> ATFEIVNRCSYTVWAAASKGDAALDAGGRQLNSGESWTINVEPGTNGGKIWARTDCYFDDSGSGICKTGDCGGLLRCKRFGRPPTTLAEFSLNQYGKDYIDISNIKGFNVPMDFSPTTRGCRGVRCAADIVGQCPAALKAPGGGCNDACTVFQTSEYCCTTGKCGPTEYSRFFKRLCPDAFSYVLDKPTTVTCPGSSNYRVTFCPTA

Among the sweet-tasting proteins, thaumatin is ~100,000 times sweeter than sucrose on a molar basis and about 1,600 times sweeter on a weight basis. The intensely sweet taste of thaumatin has been widely used not only as a natural sweetener, but also as a flavor enhancer and for masking unpleasant tastes in the food and pharmaceutical industries. Site-directed mutagenesis studies revealed that six lysine residues of Lys19, Lys49, Lys67, Lys106, Lys163, and Lys187, and three arginine residues of Arg76, Arg79, and Arg82 located on the cleft-containing side are responsible for sweetness, and two amino acids residues, Lys67 and Arg82, are particularly important for sweetness. In the present study, three mutant X-ray crystallographic structures of thaumatin (K78A, K106A, and K137A) were determined at resolutions of 1.07, 1.07 and 1.01 Å, respectively.

The final model of K137A thaumatin was determined at a slightly higher resolution of 1.01 Å. It consists of 3,309 protein atoms, including hydrogen atoms, 10 tartrate atoms, 18 glycerol atoms and 363 water molecules. Compared to K78A, K106A, and recombinant thaumatin, one tartrate molecule was reduced in K137A. The threshold values of K78A and K137A were 220 and 230 nM, respectively, and sweetness decreased by ~5-fold when compared to recombinant and plant thaumatin. In Lys137 of recombinant thaumatin, the B-factors of the main-chain and side-chain were 9.33 and 32.24 Å2, respectively. The normalized B-factor ratios of Ala137 were 1.00 for main-chain and 1.18 for side-chain, and those of Lys137 in recombinant thaumatin for main-chain and side-chain were 0.95 and 2.27, respectively. The normalized B-factor ratio decreased by 1.09 for side-chain, suggesting that the flexibility of the side-chain of Lys137 was substantially reduced. The reduction of flexibility at the interaction sites indeed seems to be consistent with the difference in sweetness, since the threshold value of K137A (230 nM) and K78A (220 nM) is higher than that of K106A (140 nM). The superposition between K137A and recombinant thaumatin showed no obvious differences in r.m.s.d. values except alternative side-chains and C-terminal Ala207 as with K78A and K106A. Three lysine residues (Lys78, Lys106, and Lys137) are still tightly interacting with the negatively charged residues on the sweet receptor, that is, NZ of Lys78 is 4.5 Å from CG of Asp433_T1R2, NZ of Lys137 is 5.0 Å from CB of Asp215_T1R3, and NZ of Lys106 interact with CG of Asp173_T1R2, suggesting all these tight interactions reflect a good complementarity.> MQTDTSNRLKQIMAE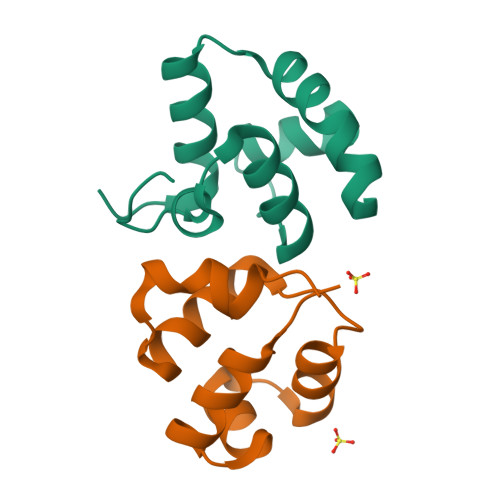RNLKQVDILNLSIPFQKKFGIKLSKSTLSQYVNSVQSPDQNRIYLLAKTLGVSEAWLMGFDVPMVESSKIENDSHHHHHH;> GSMSYDYSSLLGKITEKCGTQYNFAIAMGLSERTVSLKLNDKVTWKDDEILKAVHVLELNPQDIPKYFFNAKVH> SPSAEACGYSDRVAQLTIGNSTITTQEAANIIVGYGEWPSYC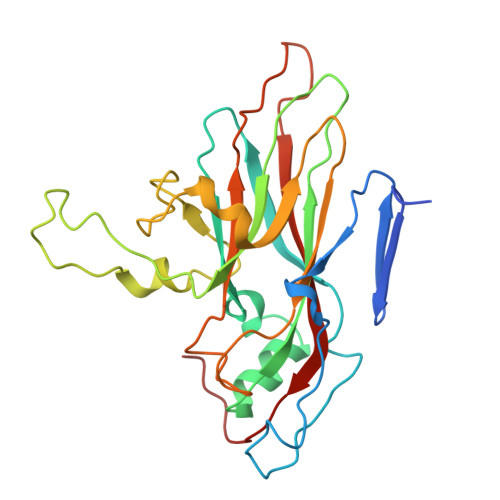SDDDATAVDKPTRPDVSVNRFYTLDTKLWEKSSKGWYWKFPDVLTETGVFGQNAQFHYLYRSGFCIHVQCNASKFHQGALLVAILPEYVIGTVAGGTGTEDSHPPYKQTQPGADGFELQHPYVLDAGIPISQLTVCHHQRINLRTNNCATIIVPYMNTLPFDSALNHCNFGLLVVPISPLDFDQGATPVIPITITLAPMCSEFAGLRQAVTQ> MAHAGRTGYDNREIVMKYIHYKLSQRGYEWDAGDDVEENRTEAPEGTESEVVHLTLRQAGDDFSRRYRRDFAEMSSQLHLTPFTARGRFATVVEELFRDGVNWGRIVAFFEFGGVMCVESVNREMSPLV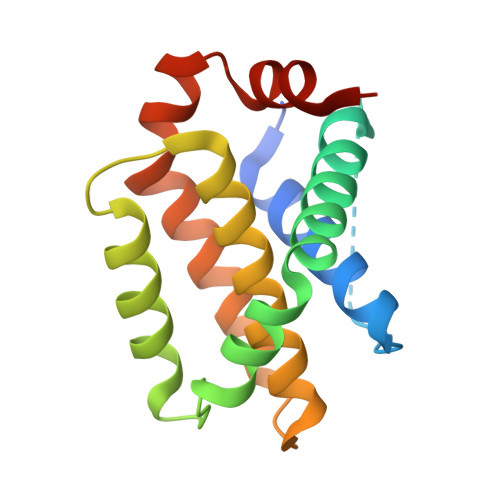DNIALWMTEYLNRHLHTWIQDNGGWDAFVELYGPSMR> GA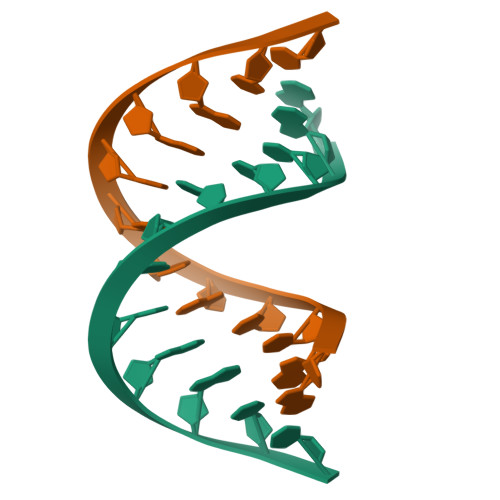CCACGTGGTC> SVAILQKRDHEGFGFVLRGAKAETPIEEFTPTPAFPALQYLESVDVEGVAWKAGLRTGDFLIEVNGVNVVKVGHKQVVGLIRQGGNRLVMKV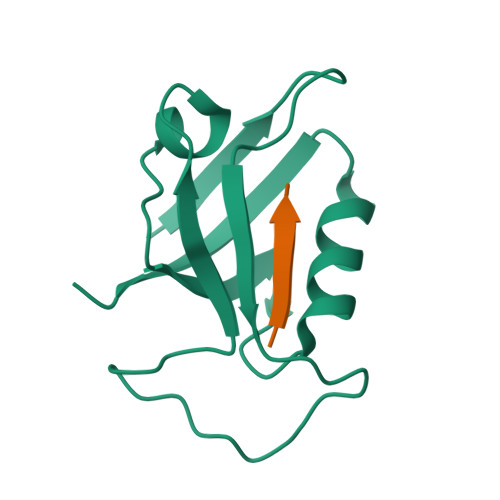VSVT;> XQLVTSL>[4x]AEEFPVPNGFESAYRE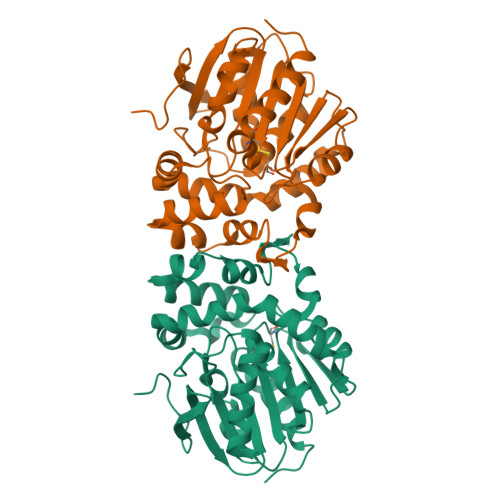VDGVKLHYVKGGQGPLVMLVHGFGQTWYEWHQLMPELAKRFTVIAPDLPGLGQSEPPKTGYSGEQVAVYLHKLARQFSPDRPFDLVAHSIGIWNTYPMVVKNQADIARLVYMEAPIPDARIYRFPAFTAQGESLVWHFSFFAADDRLAETLIAGKERFFLEHFIKSHASNTEVFSERLLDLYARSYAKPHSLNASFEYYRALNESVRQNAELAKTRLQMPTMTLAGGGHGGMGTFQLEQMKAYAEDVEGHVLPGCGHWLPEECAAPMNRLVIDFLSRGRHHHHHH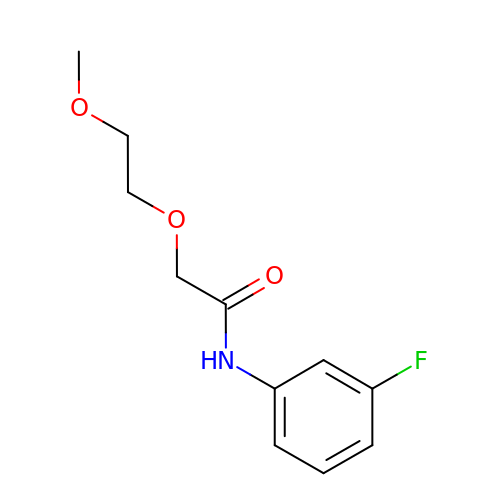N-(3-fluorophenyl)-2-(2-methoxyethoxy)acetamide | C11 H14 F N O3 | DGGIZNHJWLTAAM-UHFFFAOYSA-N> MPFTIDSARGIFPN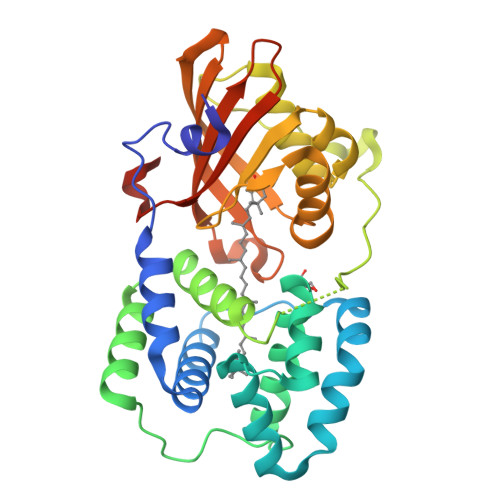TLAADVVPATIARFSQLNAEDQLALIWFAYLEMGKTLTIAAPGAASMQLAENALKEIQAMGPLQQTQAMCDLANRADTPLCRTYASWSPNIKLGFWYRLGELMEQGFVAPIPAGYQLSANANAVLATIQGLESGQQITVLRNAVVDMGFTAGKDGKRIAEPVVPPQDTASRTKVSIEGVTNATVLNYMDNLNANDFDTLIELFTSDGALQPPFQRPIVGKENVLRFFREECQNLKLIPERGVTEPAEDGFTQIKVTGKVQTPWFGGNVGMNIAWRFLLNPEGKIFFVAIDLLASPKELLNFARHHHHHH> MASTGETTYKKTTSSALKGAIQLGITHSVGSLSQKPERDVLMQDFEVVESIFFPSQGSSSTPGHHHGDFKFKTYAPIAFRYFREMFGIRPDDYLYSLCNEPLIELSNPGASGSLFYVSSDDEFIIKTVQHKEAEFLQTLLPGYFMNLNQNMRTLLPKFYGLYCVQADGKNIRIVVMNNLLPRAVPMHLKFNLKGSTYKRRASPKERSKGVPTYKDLDFMQDMPEGILLENDHYTALSRTMQRDCRVLQSFKIMDYSLLVGIHILHRAGEEASTAVPDTQKKGQGQKPLYCT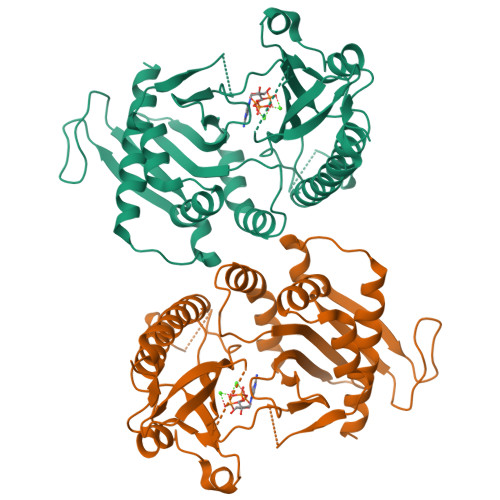AIESIQGESKSKTSPQPYESMGGIPAFNSKGERLLVFIGIIDILQSYRLVKKLEHSWKALLHDGDTVSVHRPSFYADRFQKFMCSTVFRKSQLKTLEHHHHHH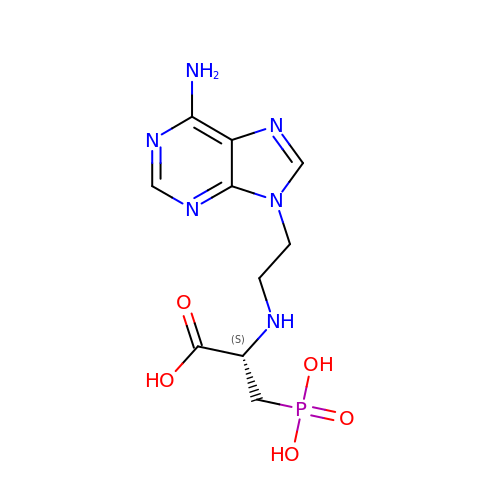(S)-2-((2-(6-amino-9H-purin-9-yl)ethyl)amino)-3-phosphonopropanoic acid | C10 H15 N6 O5 P | RZABPFHILMTNTM-ZCFIWIBFSA-N Quinol-dependent nitric oxide reductases (qNORs) are considered members of the respiratory heme-copper oxidase superfamily, are unique to bacteria, and are commonly found in pathogenic bacteria where they play a role in combating the host immune response. qNORs are also essential enzymes in the denitrification pathway, catalysing the reduction of nitric oxide to nitrous oxide. Located in the cytoplasmic membrane, NORs reduce the NO produced by nitrite reductase and catalyze N—N bond formation in the reaction 2NO + 2H+ + 2e- → N2O + H2O with the formation and release of nitrous oxide (N2O). In contrast, qNORs are single subunit enzymes (NorZ) which use membrane-bound quinol as an electron source. Whilst cNOR is predominantly found in denitrifying organisms, qNORs are also found in several pathogenic bacteria, where the enzyme detoxifies NO produced by the host’s immune response.

Here, we report a high resolution, 2.2 Å, structure of AxqNOR. The overall fold revealed 18 α-helices packed together into each monomer, with residues 113–122, 227–255, and 564–571, creating the dimer interface. In our structure, the Ca ion is ligated by seven oxygen atoms, OH Tyr78, O Gly76, OE2, and OE2 Glu407, single oxygens from propionates of heme b and heme b3 and a water molecule. In the map presented here, a weak density corresponding to a non-protein molecule is visible away from the transmembrane domain close to Asp724 and His305. We propose that the density in our map likely corresponds to an endogenous electron donor that was likely carried through from the E. coli in which the protein was expressed, since no such molecule or analog was added during sample preparation. Residues Glu309 and Arg720 are hydrogen bonded to the ubiquinol ligands His305 and Asp724, respectively, with a critical Arg720 also making a stacking interaction with heme b, positioning it favorably for electron transfer. Analysis of our cryoEM structure of AxqNOR and that of PacNOR(7) has highlighted an attractive alternative route for NO entry, which is also compatible with binding the cognate partner protein CuNiR during turnover (indicated by red arrows). The conformation of Glu490, the gatekeeper of channel entry from the catalytic site, is different from the previously reported structure. Here, it is hydrogen bonded to the bridging hydroxyl and W2, in contrast to being previously directed into the channel and hydrogen bonded with Glu5599.

>[2x]MGPYRRLWFTLIAVLAVTFALLGFYGGEVYRQAPPIPEEVASADGTRLFGRDDILDGQTAWQSIGGMQLGSIWGHGAYQAPDWTADWLHRELMAWLDLAARDAHGRDYGQLDAPAQAALREQLKAEYRANRADAAGGKLTLSPRRAQAVAQTEAYYDQLFSDAPALHRSRENYAMKENTLPDANRRRQMTHFFFWTAWAAATEREGTSVTYTNNWPHEPLIGNHPSSENVMWSIISVVVLLAGIGLLIWAWAFLRGKEEDEPPAPARDPLTTFALTPSQRALGKYLFLVVALFGFQVLLGGFTAHYTVEGQKFYGIDLSQWFPYSLVRTWHIQSALFWIATGFLAAGLFLAPLINGGRDPKYQKAGVDILFWALVLVVVGSFAGNYLAIAQIMPPDLNFWLGHQGYEYVDLGRLWQIGKFAGICFWLVLMLRGIVPALRTPGGDKNLLALLTASVGAIGLFYGAGFFYGERTHLTVMEYWRWWIVHLWVEGFFEVFATTALAFIFSTLGLVSRRMATTASLASASLFMLGGIPGTFHHLYFAGTTTPVMAVGASFSALEVVPLIVLGHEAWENWRLKTRAPWMENLKWPLMCFVAVAFWNMLGAGVFGFMINPPVSLYYIQGLNTTPVHAHAALFGVYGFLALGFTLLVLRYIRPQYALSPGLMKLAFWGLNLGLALMIFTSLLPIGLIQFHASVSEGMWYARSEAFMQQDILKTLRWGRTFGDVVFLLGALAMVVQVILGLLSGKPAAAEPVLRAEPARR Fragile X syndrome (FXS) is a genetic disorder caused by an expansion of CGG/CCG tandem repeats in the Fragile X Mental Retardation 1 gene (FMR1) on the X chromosome. Recently, our studies have suggested that the expansion of (CCG)n trinucleotide repeats (TNRs) may be attributed to the slippage of DNA strands along the hairpin structures, forming a four-stranded helical structure that is stabilized by intertwining i-motifs during DNA replication. Chromomycin A3 (Chro), produced by some strains of Streptomyces griseus, is an anthraquinone glycoside antibiotic belonging to the aureolic acid family. In the presence of divalent cobalt ions, Chro can also form a metal-coordinated dimer CoII(Chro)2, which binds selectively to GpC sequences in the minor groove of DNA.

The electron density map with a resolution of 1.87 Å revealed that all atoms in the refinement structure had a clear electron density, except for two cytosines (C2 and C13), which were extruded from the structure due to poor mapping and had to be modelled with an energy minimization module using Accelrys Discovery Studio Client (v2.5.0.9164). CoII(Chro)2 bound to the pseudo-palindromic duplex DNA sequence in the minor groove, resulting in the formation of a CoII(Chro)2-d[T(CCG)3A]2 complex. A central d(GGCC) motif was formed due to the extrusion of four cytosines (C5, C6, C16, and C17) upon binding to a Chro dimer. Unlike the i-motif adopted by dT(CCG)3A dimeric hairpins, the guanine base of the second CCG unit of each DNA strand was not flipped out, resulting in the re-formation of a GGCC tetranucleotide tract that provided the flexibility in the DNA to better accommodate CoII(Chro)2. The four projected cytosines (C5, C6, C16, and C17) interacted with the disaccharide B ring of (Chro)2 so as to enhance the stability of the extruded residues via hydrogen bonds and van der Waals forces. There were three cobalt ions (Co1, Co2, and Co3) present in the CoII(Chro)2-d[T(CCG)3A]2 complex. The Co1 ion formed an octahedral coordination with two oxygen atoms, O1 and O9, of each chromophore moiety and two oxygen atoms of water in the centre of the (Chro)2 complex. In the major groove, the Co2 and Co3 ions interacted with N7 of guanine G7 and G18, also forming an octahedral coordination with guanine and five water molecules. Based on these interactions, it can be concluded that the inclusion of Co(II) is crucial for maintaining the CoII(Chro)2-d(T(CCG)3A)2 complex structure. In addition, we found that specific binding of CoII(Chro)2 to d(CCG)n sequences induced conformational changes of the CCG repeat DNA from i-motif to DNA duplex with cytosine-cytosine flip out.

>TCCGCCGCCGA[2x]3,4,5,6-tetrahydro-2,3'-bipyridine | 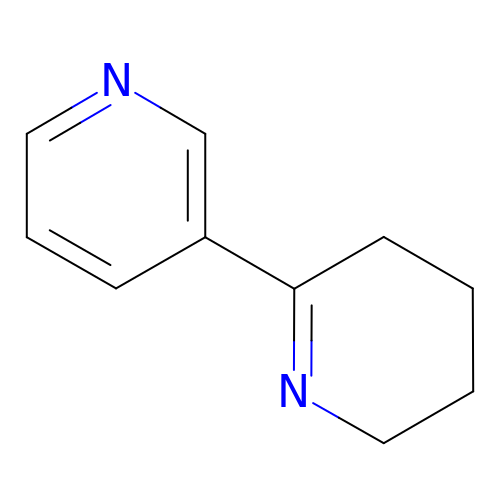C10 H12 N2 | AUBPMADJYNSPOA-UHFFFAOYSA-N>GSFSKEESREFMAIFPDIVRDLTDAGRHTDIPEVTKRFAKVLQYNVPTGKKTRGLSTVIAYKMLEKPENLTPENVRLAGILGWCVELLQASLLIMDDLMDRSETRRGQPCWYRQENVGFLAINDCLHVESSLYSVLRKYFSHLPCYVPIIELFHDVNFKTNMGQSLDALCMKDGRPILSQFTMKRYSSIVKYKTSYYTFQLPVSLGMYLADMYDPEQHRQAKTILMEIGEFFQIQDDFLDAFGDSQVTGKVGTDIKEGKCSWLAVVALQRSNPAQRQIMEEHYGRPEPESTQIIKNLYIELGLPATFAVYEEESFNIIRTHIHQISKGLPHDLFFKIMKKIYKRDA[6x]

Here we characterize a metal-dependent, bifunctional isoprenyl diphosphate synthase from the leaf beetle Phaedon cochleariae by structural and functional analyses. Isoprenyl diphosphate synthase in P. cochleariae (PcIDS1, EC 2.5.1.1) produces FPP in the presence of Mg2+, but preferably forms GPP when exposed to the heavy metal ions (HMIs) Co2+ or Mn2+. Inter- and intramolecular cooperative effects in the homodimer strongly depend on the provided metal ions and regulate the biosynthetic flux of terpene precursors to either biological defence or physiological development. Strikingly, a unique chain length determination domain adapts to form geranyl or farnesyl pyrophosphate by altering enzyme symmetry and ligand affinity between both subunits.

Remarkably, the three metal positions depict a uniform anomalous density for Mn2+ despite a 100-fold Mg2+ excess in the crystallization buffer. Thus, in the absence of IPPHAl, the staggered configuration of PPAl selects for Mn2+A and Mn2+C. Once IPP coordinates the HAl site, the high affinity of Mn2+ replaces Mg2+B and stabilizes the eclipsed orientation of PPAl, driving PPi release. So far, the described Mn2+-bound complexes all form symmetric homodimers with ligands at both Al and HAl sites. In addition, with either IPPHAl or DMAPPHAl, HMIs abolish Mg2+D coordination at PPAl and enhance GPP formation.>[7x]ADSDINIKTGTTDIGSNTTVKTGDLVTYDKENGMHKKVFYSFIDDKNHNKKLLVIRTKGTIAGQYRVYSEEGANKSGLAWPSAFKVQLQLPDNEVAQISDYYPRNSIDTKEYMSTLTYGFNGNVTGDDTGKIGGLIGANVSIGHTLKYVQPDFKTILESPTDK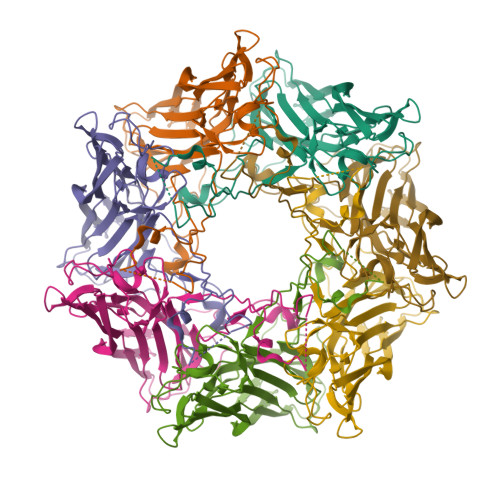KVGWKVIFNNMVNQNWGPYDRDSWNPVYGNQLFMKTRNGSMKAADNFLDPNKASSLLSSGFSPDFATVITMDRKASKQQTNIDVIYERVRDDYQLHWTSTNWKGTNTKDKWTDRSSERYKIDWEKEEMTN> MEQEKAVTDMDINELRKLMIGKAIINSSDMQGDLLQEAQDVIQSGIENNSAPVLNIEAACKYIKENLDKKFGPTWQ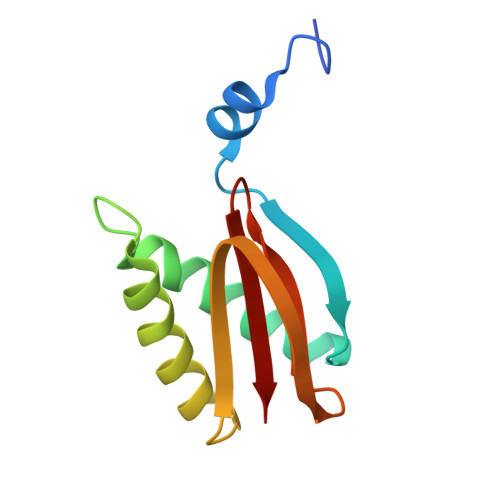CIIGEGYAYDVTVQNNTLLFMFYNGNLAVLIFKS> GPDSMVLLSSSWLPLNKDIEVEVVDYLPSSSVAPDLFALTLLRINDSSMKEKYDSMHEKMNAYAQIVPFDSELEIGYDGVFRDAPRSVRRVRRISATKLYLVDFGKIINYEKAKCFQLPKVFQSMPTRVSLCGLDGLTWSPVAIPSFDNIREVVKKWGQMENSTLHAMACGFQGSINMINLFCGKSILADRLQRKGVCEYL;> GPDSMEVEESLLDALLGKALAGDQMNSRIEGLFEDLD

Here, we identify an endoribonuclease, precursor of 21U RNA 5′-end cleavage holoenzyme (PUCH), that initiates piRNA processing in the nematode Caenorhabditis elegans. Genetic and biochemical studies show that PUCH, a trimer of Schlafen-like-domain proteins (SLFL proteins), executes 5′-end piRNA precursor cleavage. We also demonstrate how PUCH interacts with PETISCO, a complex that binds to piRNA precursors, and that this interaction enhances piRNA production in vivo.

If PUCH cleaves PETISCO-bound precursors, interactions between the two complexes may be expected. Using a combination of pull-down and size-exclusion chromatography experiments, we narrowed down the interaction to a region upstream of the TOFU-1 SLFN domain (residues 82–172, TOFU-1N) and to the extended TUDOR (eTUDOR) domain of the PETISCO subunit TOFU-6 (TOFU-6eTUDOR). AlphaFold predictions showed two helices in the N-terminal part of TOFU-1, and a construct containing only the first helix (residues 82–113, TOFU-1pep) was sufficient to bind to TOFU-6eTUDOR. Quantitative analysis with the minimal TOFU-1pep using isothermal titration calorimetry revealed a Kd of around 20 μM. We determined the crystal structure of the TOFU-6eTUDOR–TOFU-1pep complex at a resolution of 2.2 Å. On the basis of the interaction interface, we designed mutations in both TOFU-1pep and TOFU-6eTUDOR that should disrupt their interaction and tested these using pull-downs and size-exclusion chromatography. Whereas mutations on only one of the partners (especially TOFU-1pep) weakened the interaction, mutation of both partners fully disrupted the interaction. We next tested the same mutations in vivo, using CRISPR–Cas9-mediated mutagenesis of the endogenous loci. Sequencing of piRNAs and their precursors from both single and double mutants revealed a reduction in mature piRNAs, as well as an accumulation of precursors. We conclude that piRNA accumulation in vivo is stimulated by the interaction between PETISCO and PUCH.> IKGGLFADIASHPWQAAIFAKHRRSPGERFLCGGILISSCWILSAAHCFQERFPPHHLTVILGRTYRVVPGEEEQKFEVEKYIVHKEFDDDTYDNDIALLQLKSDSSRCAQESSVVRTVALPPADLQLPDWTECELSGYGKHEALSPFYSERLKEAHVRLYPSSRCTSQHLLQRTVTDNMLCAGDTRSGGPQANLHDACQGDAGGPLVCLNDGRM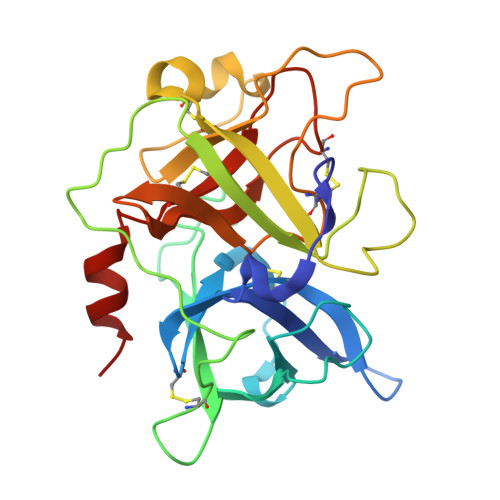TLVGIISWGLGCGQKDVPGVYTKVTNYLDWIRDNMRP> GSAMRSAQVYRWQIPMDAGVVLRDRRLKTRDGLYVCLREGEREGWGEISPLPGFSQETWEEAQSVLLAWVNNWLAGDCELPQMPSVAFGVSCALAELTDTLPQAANY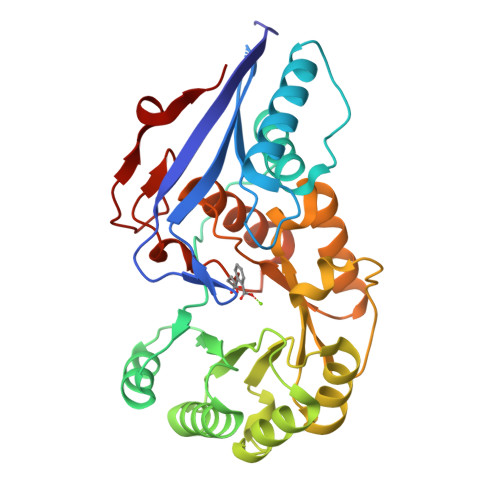RAAPLCNGDPDDLILKLADMPGEKVAKVKVGLYEAVRDGMVVNLLLEAIPDLHLRLDANRAWTPLKGQQFAKYVNPDYRDRIAFLEEPCKTRDDSRAFARETGIAIAWDESLREPDFAFVAEEGVRAVVIKPTLTGSLEKVREQVQAAHALGLTAVISSSIESSLGLTQLARIAAWLTPDTIPGLDTLDLMQAQQVRRWPGSTLPVVEVDALERLL>[2x]GPHMEDRAAQSLLNKLIRSNLVDNTNQVEVLQRDPNSPLYSVKSFEELRLKPQLLQGVYAMGFNRPSKIQENALPLMLAE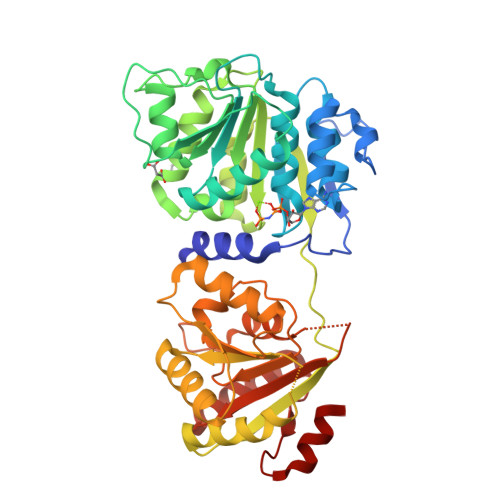PPQNLIAQSQSGTGKTAAFVLAMLSQVEPANKYPQCLCLSPTYELALQTGKVIEQMGKFYPELKLAYAVRGNKLERGQKISEQIVIGTPGTVLDWCSKLKFIDPKKIKVFVLDEADVMIATQGHQDQSIRIQRMLPRNCQMLLFSATFEDSVWKFAQKVVPDPNVIKLKREEETLDTIKQYYVLCSSRDEKFQALCNLYGAITIAQAMIFCHTRKTASWLAAELSKEGHQVALLSGEMMVEQRAAVIERFREGKEKVLVTTNVCARGIDVEQVSVVINFDLPVDKDGNPDNETYLHRIGRTGRFGKRGLAVNMVDSKHSMNILNRIQEHFNKKIERLDTDDLDEIEKIAN> KETAAAKFERQHMDSSTSAASSSNYCNQMMKSRNLTKDRCKPVNTFVHESLADVQAVCSQKNVACKN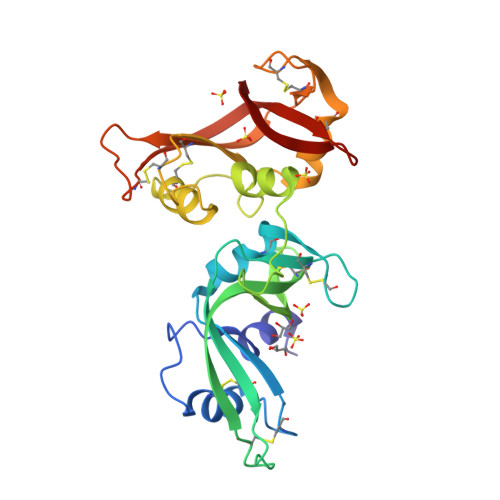GQTNCYQSYSTMSITDCRETGSSKYPNCAYKTTQANKHIIVACEGNPYVPVHFDASVSGRSGRSGKETAAAKFERQHMDSSTSAASSSNYCNQMMKSRNLTKDRCKPVNTFVHESLADVQAVCSQKNVACKNGQTNCYQSYSTMSITDCRETGSSKYPNCAYKTTQANKHIIVACEGNPYVPVHFDASV>MGRLRRRQEIIDHEEEESNDDVSSRRGKLSLAETFRWLDSSEHRRIETDGHNDYKYIIHPKNRWYKAWEMFILVWAIYSSLFTPMEFGFFRGLPERLFVLDIVGQIAFLVDIVLQFFVAYRDTQTYRTVYKPTRIAFRYLKSHFLMDFIGCFPWDLIYKASGKHELVRYLLWIRLFRVRKVVEFFQRLEKDTRINYLFTRILKLLFVEVYCTHTAACIFYYLATTLPPENEGYTWIGSLKLGDYSYENFREIDLWKRYTTALYFAIVTMATVGYGDIHAVNLREMIFVMIYVSFDMVLGAYLIGNITALIVKGSNTERFRDKMNDLISFMNRKKLGRDLRSQITGHVRLQYDSHYTDTVMLQDIPASIRAKIAQLLYLPYIKKVPLFKGCSTEFINQIVIRLHEEYFLPGEVITEQGNVVDHLYFVCEGLLEALVTKTDGSEESVTLLGPHTSFGDISIICNISQPFTVRVCELCHLLRLDKQSFSNILEIYFHDGRTILNNIMEEKESNDRIKKLESDIVIHIGKQEAELALKVNSAAFQGDFYQLKSLIRSGADPNKTDYDGRSPLHLAACRGYEDITLFLIQEGVDVNLKDKFGHTPLFEAVKAGQEGVIGLLVKEGASFNLEDSGNFLCTTVAKGDSDFLKRLLSSGMNPNSEDYDHRTPLHVAASEGLFLMAKMLVEAGASVISKDRWGNSPLDEARLCGNKKLIKLLEDVKNAQSSIYPSSLRELQEERIERRKCTVFPFHPQEAKEERSRKHGVVVWIPSNLEKLIVTAAKELGLSDGASFVLLSEDQGRITDIDMISDGHKLYMISDTTDQT[4x]

GORK is a shaker-like potassium channel in plants that contains ankyrin (ANK) repeats. GORK, also known as guard cell outward rectifying K+ channel, is the only outward-rectifying potassium channel in guard cells. In contrast, GORK activation causes potassium efflux, reducing guard cell turgor and volume and in turn stomatal closure. Each protomer has an N-terminal transmembrane domain (TMD, residues 58–313, containing helices S1–S6), followed by three cytoplasmic domains: the C-linker (residues 314–365), cyclic nucleotide-binding domain homolog (CNBDH) (residues 366–510), and ANK (residues 511–724).

Tetrameric reconstructions of AtGORK were obtained in two conformational states at resolutions of 3.4 Å (AtGORKFL1) and 4.3 Å (AtGORKFL2), allowing de novo modeling of 662 of 820 amino acids (residues 58–720) for each protomer, while the remaining regions were not resolved due to their intrinsic flexibility. The full-length AtGORKFL forms a tetramer with elongated cytoplasmic regulatory domains, with its architecture showing a symmetry reduction from four-fold (C4) to two-fold (C2). Remarkably, ANK repeats from two neighboring protomers form a stable dimer through specific interactions mediated by their protruding loops, creating a buried area of ~1,500 Å2. This dimeric interaction is specific, corroborated by another structure of the full-length of AtGORKFL2, which retains similar dimeric units despite of variation in their tetrameric conformations. Our structural studies reveal that ANK dimerization in full-length AtGORK is directly responsible for reducing its tetrameric symmetry from C4 to C2, maintaining an autoinhibited state. Thus, the current AtGORK structure likely represents an autoinhibited, preactivation state.>SAFDQAARSRGHNNRRTALRPRRQQEATEVRPEQKMPTLLRVYIDGPHGMGKTTTTQLLVALGSRDDIVYVPEPMTYWRVLGASETIANIYTTQHRLDQGEISAGDAAVVMTSAQITMGMPYAVTDAVLAPHIGGEAGSSHAPPPALTLIFDRHPIAALLCYPAARYLMGSMTPQAVLAFVALIPPTLPGTNIVLGALPEDRHIDRLAKRQRPGERLDLAMLAAIRRVYGLLANTVRYLQCGGSWREDWGQLSGTAVPPQG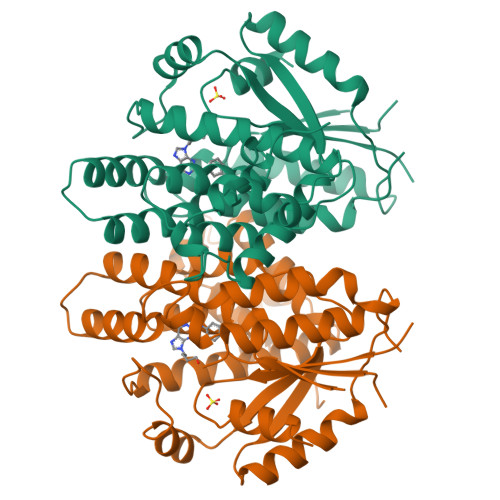AEPQSNAGPRPHIGDTLFTLFRAPELLAPNGDLYNVFAWALDVLAKRLRSMHVFILDYDQSPAGCRDALLQLTSGMVQTHVTTPGSIPTICDLARTFAREMGEAN[2x]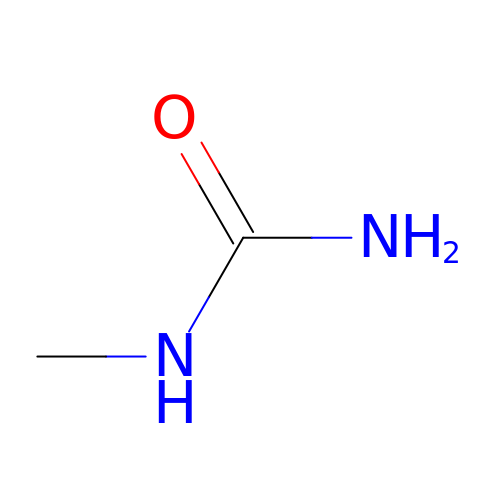N-METHYLUREA | C2 H6 N2 O | XGEGHDBEHXKFPX-UHFFFAOYSA-N> GPSLDFALSLLRRNIRQVQTDQGHFT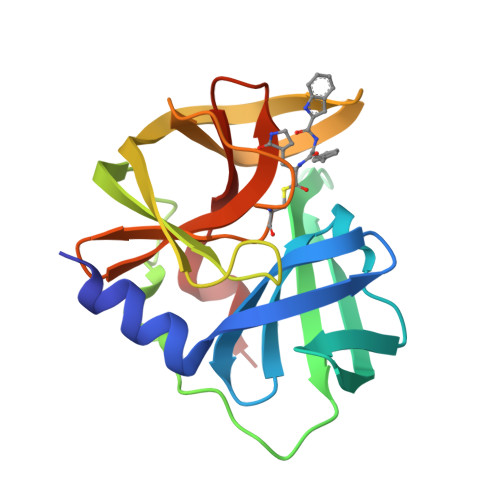MLGVRDRLAVLPRHSQPGKTIWVEHKLVSVLDAVELVDEQGVNLELTLITLDTNEKFRDITKFIPENISTASDATLVINTEHMPSMFVPVGDVVQYGFLNLSGKPTHRTMMYNFPTKAGQCGGVVTSVGKVVGIHIGGNGRQGFCAGLKRSYFASEQ1-[3-(hexyloxy)benzyl]-4-hydroxy-2-oxo-1,2-dihydropyridine-3-carboxylic acid | C19 H23 N O5 | 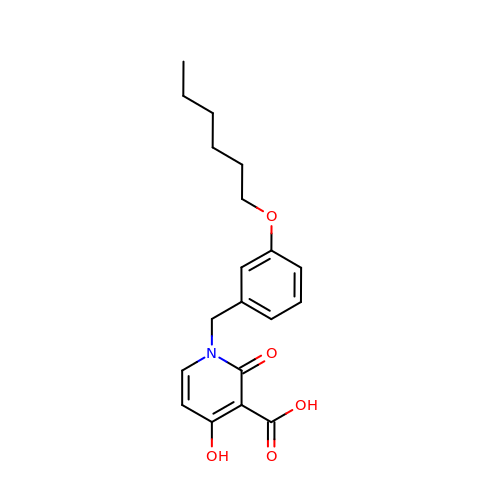IEFKPWNGVIDYEA-UHFFFAOYSA-N DIPHOSPHOMETHYLPHOSPHONIC ACID ADENYLATE ESTER | 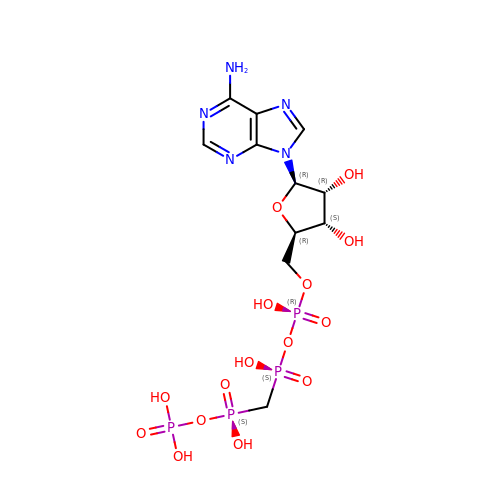C11 H19 N5 O15 P4 | ARRGHMSEJJFDME-IOSLPCCCSA-N> MMTQKKNDSNIPNYYLYGTVLTRYGLASLNHDIRRGNKTILQKGYWNNGKIHSFVGSSAIRWALRFYLQKQGYLVNRVWDEEEHINRLTSEDFDPEKFYDDDIFGFALLESAETEEDTSTTKRKKKQTKTSTPNQRMGALGMNMAVSLTPYDGAVKLGAKSGREKDSTSLHFTEYHATRYQYYFGIDATHLKDFSRILPMIDGIMNLPKVGGSSNIFNYPFCPDSLVFQWTNHFASYISYCFEYCDPKSKEAKLSQEFIDEVECGQIDPSKLWIGGTIVKDLQQLDNFESSPLNKAHIY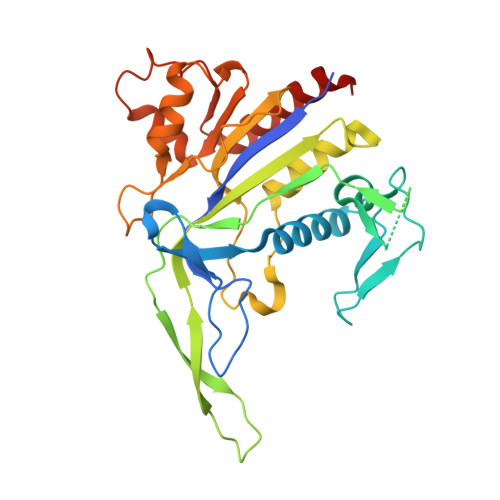RNRNEMIEALKTVIKRDLGLEESK> SMSSFEGQMAEYPTISIDRFDRENLRARAYFLSHCHKDHMKGLRAPTLKRRLECSLKVYLYCSPVTKELLLTSPKYRFWKKRIISIEIETPTQISLVDEASGEKEEIVVTLLPAGHCPGSVMFLFQGNNGTVLYTGDFRLAQGEAARMELLHSGGRVKDIQSVYLDTTFCDPRFYQIPSREECLSGVLELVRSWITRSPYHVVWLNCKAAYGYEYLFTNLSEELGVQVHVNKLDMFRNMPEILHHLTTDRNTQIHACRHPKAEEYFQWSKLPCGITSRNRIPLHIISIKPSTMWFGERSRKTNVIVRTGESSYRACFSFHSSYSEIKDFLSYLCPVNAYPNVIPVGTTMDKVVEILKPLCRS

Artemis (SNM1C/DCLRE1C) is an endonuclease that plays a key role in development of B- and T-lymphocytes and in dsDNA break repair by non-homologous end-joining (NHEJ). Artemis is phosphorylated by DNA-PKcs and acts to open DNA hairpin intermediates generated during V(D)J and class-switch recombination. Artemis belongs to a superfamily of nucleases containing metallo-β-lactamase (MBL) and β-CASP (CPSF-Artemis-SNM1-Pso2) domains. The overall fold of the catalytic core of Artemis is similar to that of SNM1A and SNM1B (2 Å backbone RMSD); it has all the key structural characteristics of human MBL fold nucleases, with the di-metal containing active site at the interface between the MBL and β-CASP domains.

The results show that neither cefotaxime nor 7-aminocephalosporanic acid inhibit Artemis, whilst ceftriaxone inhibits with a modest IC50 of 65 μM. We solved a structure of ceftriaxone bound to Artemis (purified by IMAC) at 1.9 Å resolution in the space group P1 with one protein molecule in the asymmetric unit. As before, in this structure Artemis possesses the canonical bilobar MBL and β-CASP fold with an active site containing one nickel ion, likely reflecting the purification method. Ceftriaxone binds to the protein surface in an extended manner making interactions with the active site, towards the β-CASP domain. There is no evidence for cleavage of the β-lactam, nor of loss of the C-3′ cephalosporin side chain, reactions that can occur during ‘true’ MBL catalysed cephalosporin hydrolysis. Electron density at the active site clearly reveals the ceftriaxone side chain coordinates the M1 site nickel ion replacing two waters (72 and 106) in the uncomplexed structure. Despite the conservation of key elements of the active site of the MBL fold nucleases and the ‘true’ β−lactam hydrolysing MBLs, ceftriaxone, does not interact with the nickel ion via its β-lactam carbonyl (as occurs for the true MBLs), but via both carbonyl oxygens of the cyclic 1, 2 diamide in its sidechain (Ni–O distances: 2 and 2.2 Å), i.e. it is not positioned for productive β-lactam hydrolysis. The amino-thiazole group (N7) of ceftriaxone forms hydrogen bonds with the side chain of Asn205, while the S1 of the 7-aminocephalosporanic acid core of the compound interacts with the hydroxyl of Tyr212 through an ethylene glycol molecule. A notable difference between the ceftriaxone-bound Artemis structure and the non-complexed structure is the loss of a metal ion at M2 site, normally coordinated by Asp37, His38 and Asp130. Without a metal ion at the M2 site, as in the ceftriaxone bound structure, the Asp37 side chain is positioned away from the active site, as seen when nickel is bound in the M1 site.NVL-655 | C23 H22 Cl F N6 O | 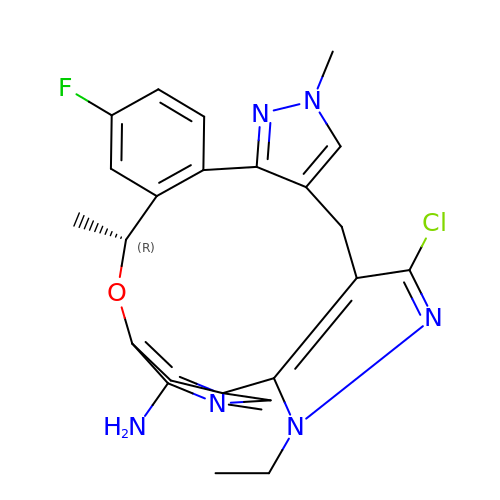FWZSCAQEBTVTOM-GFCCVEGCSA-N Bisphosphoglycerate mutase (BPGM) is an erythrocyte-specific multifunctional enzyme that is responsible for the regulation of 2,3-bisphosphoglycerate (2,3-BPG) in red blood cells through its synthase and phosphatase activities; the latter enzymatic function is stimulated by the endogenous activator 2-phosphoglycolate (2-PG). 2,3-BPG is a natural allosteric effector of hemoglobin (Hb) that is responsible for decreasing the affinity of Hb for oxygen to facilitate tissue oxygenation. BPGM is a multifunctional enzyme, functioning as a 2,3-BPG synthase, a 2,3-BPG phosphatase and a phosphoglycerate mutase. The phosphatase activity is responsible for the hydrolysis of 2,3-BPG to 3-phosphoglycerate (3-PGA), an intermediate in the main glycolytic pathway.

To confirm the binding mode of 2-PG to BPGM, the crystal structure of BPGM complexed with 2-PG in the absence of 2,3-BPG was also determined to 2.48 Å resolution. The overall dimeric structure is identical to that of the ternary BPGM·3-PGA·2-PG structure. Similar to the ternary BPGM·3-PGA·2-PG complex, the monomer A active site of the binary BPGM·2-PG complex was ordered, with continuous electron density from Ser2 to Val254. In contrast, monomer B was disordered, with weak or missing electron density at the C-terminus beyond Ile245 and weak or missing side-chain density for Arg100, Arg116 and Arg117. The carboxyl group of 2-PG forms hydrogen-bond interactions with the main-chain N atoms of Cys23 (2.6 Å) and Ser24 (2.5–3.5 Å) and the guanidino group of Arg100 (3.5 Å). Our ternary BPGM·3-PGA·2-PG crystal structure shows a terminal snapshot of the catalytic phosphatase activity, with one subunit undergoing catalysis by tightly binding to the substrate (fully closed conformation), while the other subunit binds 2-PG with a partially closed conformation of the active site in monomer B. The binary BPGM·2-PG crystal structure confirmed the ability of 2-PG to bind to the active site and the presence of an alternative noncatalytic binding site at the dimer interface.

>[2x]MSKYKLIMLRHGEGAWNKENRFCSWVDQKLNSEGMEEARNCGKQLKALNFEFDLVFTSVLNRSIHTAWLILEELGQEWVPVESSWRLNERHYGALIGLNREQMALNHGEEQVRLWRRSYNVTPPPIEESHPYYQEIYNDRRYKVCDVPLDQLPRSESLKDVLERLLPYWNERIAPEVLRGKTILISAHGNSSRALLKHLEGISDEDIINITLPTGVPILLELDENLRAVGPHQFLGDQEAIQAAIKKVEDQGKVKQAKKLEHHHHHH> GHMQLSHRPAETGDLETVAGFPQDRDELFYCYPKAIWPFSVAQLAAAIAERRGSTVAVHDGQVLGFANFYQWQHGDFCALGNMMV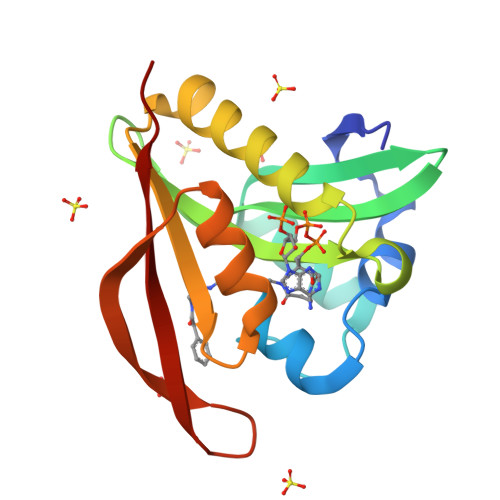APAARGLGVARYLIGVMENLAREQYKARLMKISCFNANAAGLLLYTQLGYQPRAIAERHDPDGRRVALIQMDKPLEP> GSHMSEQLTDQVLVERVQKGDQKAFNLLVVRYQHKVASLVSRYVPSGDVPDVVQEAFIKAYRALDSFRGDSAFYTWLYRIAVNTAKNYLVAQGRRPPSSDVDAIEAENFESGGALKEISNPENLMLSEELRQIVFRTIESLPEDLRMA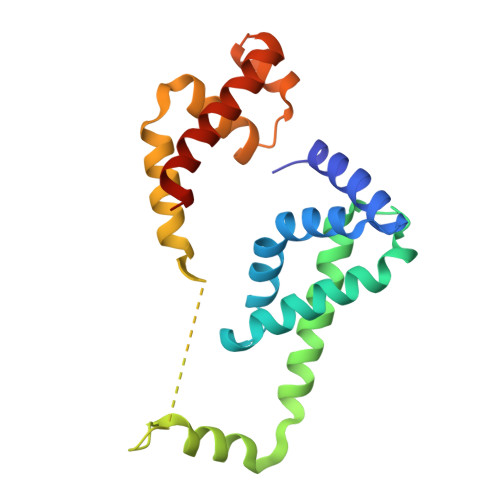ITLRELDGLSYEEIAAIMDCPVGTVRSRIFRAREAIDNKVQPLIRR> TESDRIAGIFNIPAGIIPTGNVLSTIEVCAHRCIFDFFKQIRSDDNSLYSAQFDILLGTYCNTLNFVRFLELGLSVACICTKFPELAYVRDGVIQFEVQQPMIARDGPHPVDQPVHNYMVKRIHKRSLSAAFAIASEALSLLSNTYVDGTEIDSSLRIRAIQQMARNLRTVLDSFERGTADQLLGVLLEKAPPLSLLSPINKFQPEGHLNRVARAALLSDLKRRVCADMFFMTRHAREPRLISAYLSDMVSCTQPSVMVSRITHTNTRGRQVDGVLVTTATLKRQLLQGILQIDDTAADVPVTYGEMVLQGTNLVTALVMGKAVRGMDDVARHLLDITDPNTLNIPSIPPQSNSDSTTAGLPVNARVPADLVIVGDKLVFLEALERRVYQATRVAYPLIGNIDITFIMPMGVFQANSMDRYTRHAGDFSTVSEQDPRQFPPQGIFFYNKDGILTQLTLRDAMGTICHSSLLDVEATLVALRQQHLDRQCYFGVYVAEGTEDTLDVQMGRFMETWADMMPHHPHWVNEHLTILQFIAPSNPRLRFELNPAFDFFVAPGDVDLPGPQRPPEAMPTVNATLRIINGNIPVPLCPIS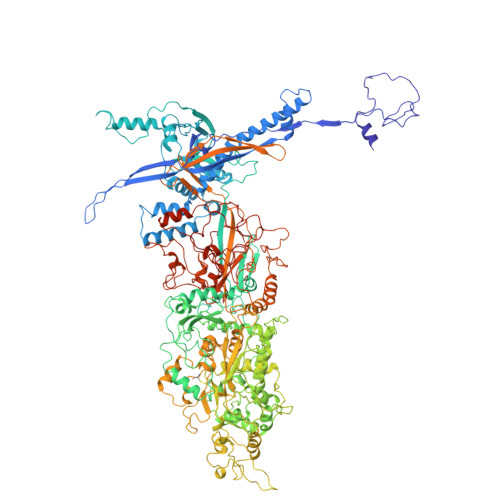FRDCRGTQLGLGRHTMTPATIKAVKDTFEDRAYPTIFYMLEAVIHGNERNFCALLRLLTQCIRGYWEQSHRVAFVNNFHMLMYITTYLGNGELPEVCINIYRDLLQHVRALRQTITDFTIQGEGHNGETSEALNNILTDDTFIAPILWDCDALIYRDEAARDRLPAIRVSGRNGYQALHFVDMAGHNFQRRDNVLIHGRPVRGDTGQAIPITPHHDREWGILSKIYYYIVIPAFSRGSCCTMGVRYDRLYPALQAVIVPEIPADEEAPTTPEDPRHPLHAHQLVPNSLNVYFHNAHLTVDGDALLTLQELMGDMAERTTAILVSSAPDAGAATATTRNMRIYDGALYHGLIMMAYQAYDETIATGTFFYPVPVNPLFACPEHLASLRGMTNARRVLAKMVPPIPPFLGANHHATIRQPVAYHVTHSKSDFNTLTYSLLGGYFKFTPISLTHQLRTGFHPGIAFTVVRQDRFATEQLLYAERASESYFVGQIQVHHHDAIGGVNFTLTQPRAHVDLGVGYTAVCATAALRCPLTDMGNTAQNLFFSRGGVPMLHDNVTESLRRITASGGRLNPTEPLPIFGGLRPATSAGIARGQASVCEFVAMPVSTDLQYFRTACNPRGRASGMLYMGDRDADIEAIMFDHTQSDVAYTDRATLNPWASQKHSYGDRLYNGTYNLTGASPIYSPCFKFFTPAEVNTNCNTLDRLLMEAKAVASQSSTDTEYQFKRPPGSTEMTQDPCGLFQEAYPPLCSSDAAMLRTAHAGETGADEVHLAQYLIRDASPLRGCLPL> ACTCGGATGAT

Here we describe the crystal structures of a DNA 11-mer that forms eight symmetric ps base pairs. Each oligonucleotide strand forms a ps duplex with a crystallographically equivalent strand, resulting in the first example of a DNA crystal structure that contains four different symmetric homo base pairs. Two of these ps duplexes are coaxially stacked in a head-to-head orientation on equivalent C–C(+) base pairs that is structurally equivalent to the stacking interactions in the DNA i-motif. Remarkably, these two duplexes are effectively locked together as a tetraplex through intercalation of the 5′-most A–A base pairs between adjacent G–G pairs in the opposite duplex.

We initially crystallized the non-derivatized DNA oligonucleotide, and utilized the BrU3 and BrU8 substitutions for phasing purposes. Though we were capable of collecting data on isomorphous native crystals, we had difficulty refining the structure despite the initial phase estimates indicating a structure very similar to the SAD-phased derivative. The native and bromine derivative crystals were isomorphous with respect to space group and unit cell dimensions, and have similar overall structures. The main difference between the native and derivative structures is the locations of extra-helical pyrimidine residues. Specifically, T3 in the native structure is not involved in the same type of crystal stacking contacts as BrU3, but is instead orientated toward the helical axis, allowing it to stack with T3 from the partner strand of the tetraplex, while also forming a hydrogen bond with C4. Additionally, C2 was nearly completely disordered in the native crystals. The lower resolution and poorer overall refinement statistics for the native structure is most likely explained by a loss of higher-order lattice structure due to the absence of these halogen interactions. We examined the native oligonucleotide by 1H NMR and native gel electrophoresis to determine if the interactions observed in the crystal structure were also present in solution. The appearance of the duplex was not greatly enhance when samples were incubated with Mg2+ higher than 50 mM. Together, the NMR and native gel analysis results strongly indicate that the oligonucleotide is capable of forming a ps duplex in solution and the NMR data suggests that the duplexes may assemble into tetraplexes.> MPKRIVYNISSDFQLKSLLGEGAYGVVCSATHKPTGEIVAIKKIEPFDKPLFALRTLREIKILKHFKHENIITIFNIQRPDSFENFNEVYIIQELMQTDLHRVISTQMLSDDHIQYFIYQTLRAVKVLHGSNVIHRDLKPSNLLINSNCDLKVCDFGLARIIDESAADNSEPTGQQSGMVEFVATRWYRAPEVMLTSAKYSRAMDVWSCGCILAELFLRRPIFPGRDYRHQLLLIFGIIGTPHSDNDLRCIESPRAREYIKSLPMYPAAPLEKMFPRVNPKGIDLLQRMLVFDPAKRITAKEALEHPYLQTYHDPNDEPEGEPIPPSFFEFDHYKEALTTKDLKKLIWNEIFS;> PRSLQN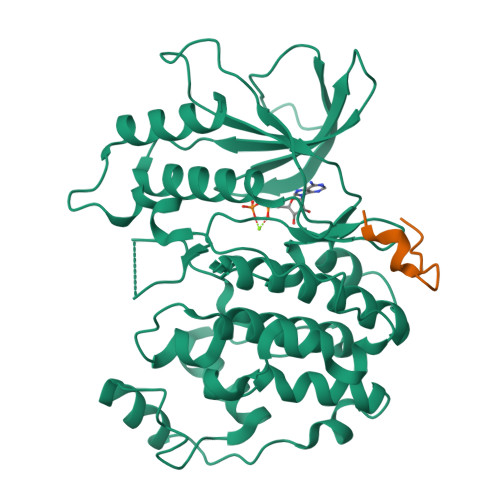RNTKNLSLDIAALHP Antascomicine B | 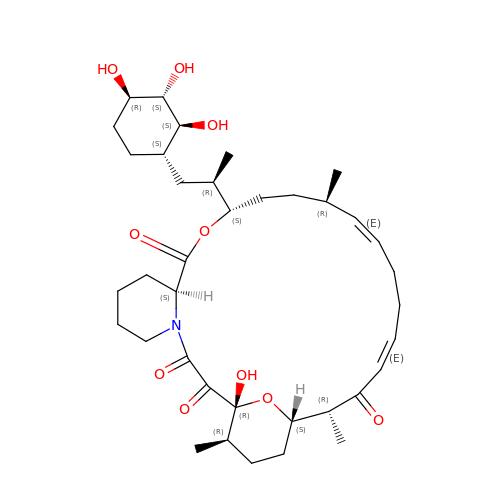C37 H57 N O10 | PSAJCYLXNSDJCJ-FALYXAMCSA-N Chlorite dismutases (Clds) are heme b-containing oxidoreductases that can decompose chlorite to chloride and molecular oxygen. The two clades exhibit differences in (i) oligomerization, with clade 1 proteins being homopenta- or homohexamers6−10 and clade 2 representatives forming homodimers,11−14 and (ii) subunit structure, with “long” clade 1 Clds being composed of an N-terminal and a C-terminal heme b-carrying ferredoxin-like domain and “short” clade 2 proteins lacking the α-helices of the N-terminal domain. The only charged amino acid in the hydrophobic distal heme cavity is a fully conserved arginine (R173 in NdCld and R127 in CCld), which is proposed to be flexible and to switch between two conformations during catalysis, i.e., pointing toward either the heme iron (“in”) or the substrate entry channel (“out”).4,6,8,11,14,16 Importantly, the hydrogen-bonding network of this catalytic arginine is different in clade 1 and clade 2 Clds. In clade 2 Clds, R127 is H-bonded to Q74 located on a flexible α-helical loop, which in general connects the N-terminal and C-terminal ferredoxin-like domains in porphyrin-binding α + β barrel proteins.

As typical for a clade 2 Cld, its distal arginine 127 is hydrogen-bonded to glutamine 74. The latter has been exchanged with either glutamate (Q74E) to arrest R127 in a salt bridge or valine (Q74V) that mirrors the setting in clade 1 Clds. The Q74V variant mirrors the situation in the clade 1 representative NdCld and should exhibit an increased flexibility of R127 compared to that of wild-type CCld, whereas Q74E might arrest the catalytic amino acid by forming a salt bridge. By contrast, in clade 1 Clds the corresponding residue [Q123 in NdCld] turns away from R173 due to a different conformation of this loop (loop colored blue). We provide the crystal structures of Q74V and Q74E and demonstrate the impact of the mutations and pH on heme coordination and active site architecture by ultraviolet–visible (UV–vis), electron paramagnetic resonance (EPR), and electronic circular dichroism (ECD) spectroscopy. Besides heme coordination, the mutations are shown to have a strong impact on the thermal stability of the heme cavity but an only weak effect on the chlorite degradation activity. The conformational dynamics of R127 is shown to have a significant role in heme coordination during the alkaline transition and in the thermal stability of the heme cavity, whereas its impact on the catalytic efficiency of chlorite degradation is relatively small.

>[2x]GPGYQDPNNRYSFIGGRTGQWQVVKIRNVLGPGLQLVEKVNILNGAVAEIPLDSAWRLQGFASNIRYAIRTELEALQAVVPMLNRAEAILAVLIPIKKSAQWWEMAQDERRDIFERESHHTAVGLEYLPGVARRLLHCRDLGEEFDFLTWFEFAPEHSSAFNELLLRMRASKEWEYVEREVEVWLKRL>MLQNSFKLAQSLRNGFYRNAWRAFSSHGPRQPLVSPERRLEKAHPTFTERSQLKYARRLVVKLGSAVITREDNHGLALGRLASIVEQVAECHLEGREVMMVTSGAVAFGKQKLAQELLMSLSMRETLNPKDSKEFDGATLEPRAAAAVGQSGLMSLYDAMFAQYGVKIAQVLVTKPDFYNEETRNNLFCTLSELISLNIVPIINTNDAVSPPMFIRDDEPAGGARRGIPIKDNDSLSAMLAAEVQADLLILMSDVDGIYNKPPWEDGAKLMHTYTSDDSNSIEFGKKSKVGTGGMDSKVKAATWALDRGVSVVICNGMQEKAIKTIIGGRKVGTFFTEATESANAVPVEVMAENARTGSRQMQALTPAQRASAVNTLADLLVSREKFILDANAKDLAEAQKSGLAKPLLSRLSLNPAKLKNLSVGLKQIAEDSHKNVGRVLRRTRLADQLELKQVTVPIGVLLVIFESRPDSLPQVAALAMASANGLLLKGGKEAAHSNKALMELVKEALATVGAEHAVS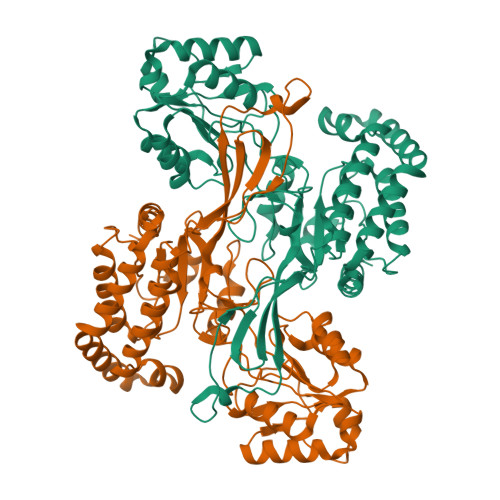LVSTREEISDLLSMENHIDLIIPRGSSDLVRSIQQQSLHIPVLGHAEGVCHVYIDRDADLEKALRIARDAKCDYPAACNAMETLLIHEDLMSGAIFGDVCNMLKREGVKIYAGPRLNQQLTFGPPAAKSLKHEYGALECCIEVVPSLDEAINHIHTYGSSHTDVIVTENDAAARQFLGSVDSACVFHNASSRFADGFRFGLGAEVGISTARIHARGPVGVEGLLTTKWILEGQDHAAADFAEGGGRTWLHETLPLD[2x]>GGSMEVGTVVQEEMKFRGSEFAVKVEMAERLLIVEISDVVTADQWRGEFGPAYIEDLTRKTGNFKQFPVFCSMLESAVHKSSDSVTL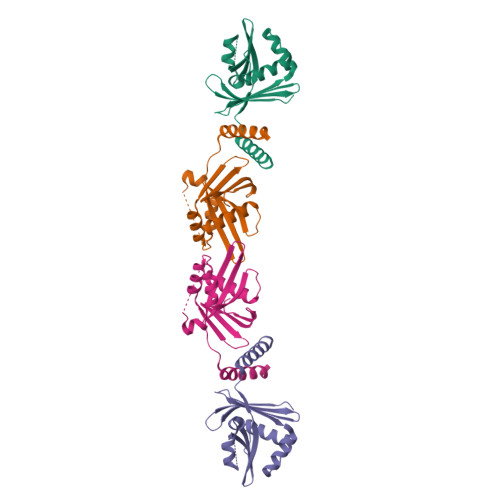DLLTYSDLELLRNRKAGVVGRPRAQPQSPALSAKRYLILIYTVEFDRIHYPLPLPYLGKPDPAELQKEIRALRSELKTLGLRGDHK[2x]>[3x]MHESVTANIENVKKVAHHIQKLTSIVPEIGIICGSGLGKLADGVKDKITIPYTKI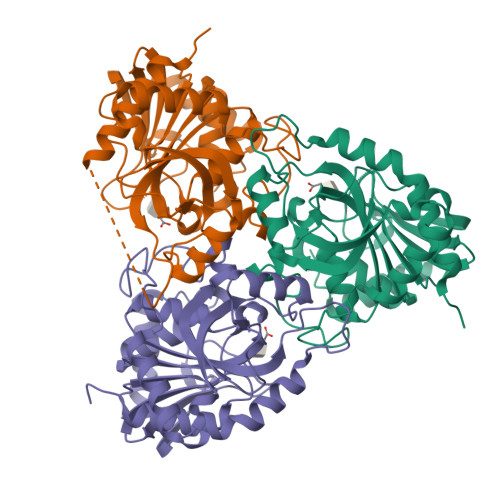PNFPQTSVVGHSGNLIFGTLSGRKVVVMQGRFHMYEGYSNDTVALPIRVMKLLGVKILMVSNAAGGLNRSLKLGDFVILKDHIYLPGLGLNNILVGPNQEAFGTRFPALSNAYDRDLRKLAVQVAEENGFGNLVHQGVYVMNGGPCYETPAECTMLLNMGCDVVGMSTIPEVVIARHCGIQVFAVSLVTNISVLDVESDLKPNHEEVLATGAQRAELMQSWFEKIIEKLPKD> GGSWEIDPKDLTF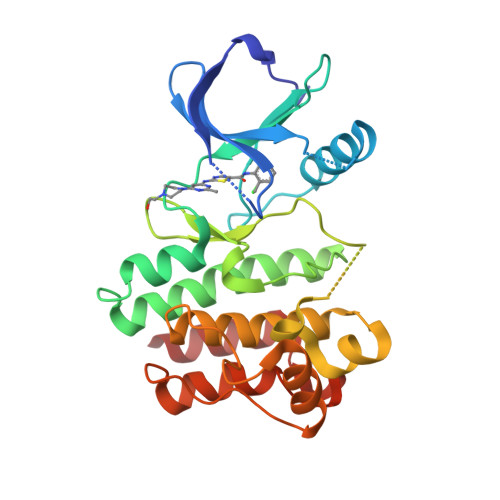LKELGTGQFGVVKYGKWRGQYDVAIKMIKEGSMSEDEFIEEAKVMMNLSHEKLVQLYGVCTKQRPIFIITEYMANGCLLNYLREMRHRFQTQQLLEMCKDVCEAMEYLESKQFLHRDLAARNCLVNDQGVVKVSDFGLSRYVLDDEYTSSRGSKFPVRWSPPEVLMYSKFSSKSDIWAFGVLMWEIYSLGKMPYERFTNSETAEHIAQGLRLYRPHLASEKVYTIMYSCWHEKADERPTFKILLSNILDVMD>[4x]MGHHHHHHENLYFQGVQKIGILGAMREEITPILELFGVDFEEIPLGGNVFHKGVYHNKEIIVAYSKIGKVHSTLTTTSMILAFGVQKVLFSGVAGSLVKDLKINDLLVATQLVQHDVDLSA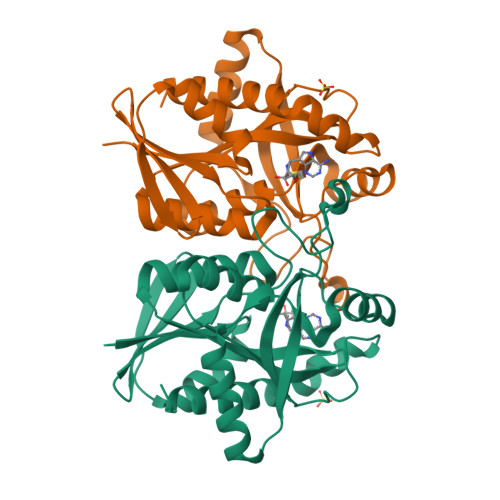FDHPLGFIPESAIFIETSGSLNALAKKIANEQHIALKEGVIASGDQFVHSKERKEFLVSEFKASAVEMEGASVAFVCQKFGVPCCVLRSISDNADEKAGMSFDEFLEKSAHTSAKFLKSMVDEL>[3x]MGIGKSPTGIQGFDELTLGGLPTGRPSLVCGSAGCGKTLFASTFLINGVRDHGEPGVFVTFEERPEDIVNNVASLGFELDKLIEEEKIAIEHIAVDPSEVAEIGDYDLEGLFLRLELAIDTVGAKRVVLDTIESLFSAFSNPAILRAEIRRLFDWLKERGLTTVITAERGDGALTRQGLEEYVSDCVILLDHRVENQISTRRLRIVKYRGTAHGTNEYPFLIDTDGFSVLPVSALGLLHQVHEERIASGVPDLDAMMAGGGFFRGSSILVSGVAGAGKSSLAAHFAAAACARGERAMYFSFEEAADQAVRNMRSLGLDLGRWRDAGLLRFMATRPTFYSLEMHLAVILREVMRFEPSVVVLDPISAFTESGDRLEVQSMLLRIVDFLKNRGITGIFTHLAHSQNEATTDAGLSSLMDGWVLMLNREVNGEFNRELYLLKARGMAHSNQVREFLMSDRGISLLPPHLGEGGALTGTARKAEEARLRRAEIE

Here we investigate the primordial circadian clock in Rhodobacter sphaeroides, which contains only KaiBC, to elucidate its inner workings despite missing KaiA. Using a combination of X-ray crystallography and cryogenic electron microscopy, we find a new dodecameric fold for KaiC, in which two hexamers are held together by a coiled-coil bundle of 12 helices. This interaction is formed by the carboxy-terminal extension of KaiC and serves as an ancient regulatory moiety that is later superseded by KaiA. Our kinetic data identify the difference in the ATP-to-ADP ratio between day and night as the environmental cue that drives the clock.

To further understand its role, we generated a truncation at residue Glu490 based on the phylogenetic tree and crystallographic information (KaiCRS-Δcoil) to disrupt the coiled-coil interaction between the two hexamers. Nucleotide exchange rates in the CII domain for KaiCRS-Δcoil and the wild-type protein were comparable (19.1 ± 0.8 h−1 and 18.0 ± 1.5 h−1, respectively). The phosphorylation rates were also similar (5.5 ± 0.4 h−1 and 7.4 ± 0.3 h−1 for KaiCRS-Δcoil and wild type, respectively). These results indicate that the extended A loop and not the coiled-coil interaction plays a pivotal part in nucleotide exchange and autophosphorylation in KaiCRS. By contrast, little dephosphorylation was observed for KaiCRS-Δcoil, for which allosteric propagation was disrupted. Consistent with this accelerated dephosphorylation rate mediated by the coiled-coil domain, our crystallographic data showed a phosphate group on Ser414 for KaiCRS-Δcoil but not for the wild-type protein. First, KaiBRS binding to either KaiCRS-CI domain or KaiCRS-Δcoil (that is, missing the C-terminal extensions) resulted in disassembly of the hexameric KaiCRS structure into its monomers.The sp0987 gene in the S. pneumoniae TIGR4 strain encodes a putative single-domain protein belonging to the GH25 family. As mutational analysis indicated that this novel protein might be involved in host-cell invasion, we named this protein Glycosyl Hydrolase 25 relating to Invasion Protein (GHIP). GHIP is a novel type of GH25 protein containing a single-domain catalytic module, which differs from other known GH25 that contain at least two distinct domains, including a catalytic module and a choline-binding module. Functionally, GHIP can hydrolyze peptidoglycan using the active site located at the mouth of its barrel structure; in addition, deleting the GHIP gene has a strongly inhibits S. pneumoniae virulence.

Therefore, in order to better understand the function of this novel virulence factor, we elucidated and now report the X-ray structure of GHIP at 1.86 Å resolution. The GHIP crystal structure was phased by single-wavelength anomalous dispersion at 3.0 Å resolution and refined against the diffraction data acquired from the native GHIP crystal at 1.86 Å with a 24.5% free R-factor and an 18.0% crystallographic R-factor. The final model consisted of 227 amino acids (residues 15–243) and 200 water molecules. Due to conformational disorder, the N-terminal residues (1–14) were not represented in the electron density and therefore not included in the final model. Only one GHIP molecule was present in the asymmetric unit. The overall structure of GHIP consists of one domain shaped into a flattened ellipsoid with dimensions of 30 Å × 38 Å × 40 Å. GHIP contains an inner ring of seven parallel β-sheets (β1–7) with a protruding β-strand (β8) at the C-terminal region, and an outer wheel composed of eight α-helices surrounds this inner ring. 14 amino acids, including Asp56, Ser58, Ser84, Tyr121, Tyr123, Glu154, Glu156, Asp157, Tyr185, Tyr209, Asp212, Ser233, Asp243, and Asp245, form a negatively charged groove at the mouth of the GHIP barrel. Analogously, the four corresponding residues in GHIP homologs, including Asp56, Asp154, Glu156, and Asp245, are also strictly conserved. All mutants showed lower hydrolytic activity compared to wild-type GHIP, suggesting that these four residues are located at the active site of this novel peptidoglycan hydrolase enzyme.

> MRKQIHPLILFSFFGIMMFILIINRPLNDSQSFKTKSNIAQIEAQALKHLDKPIIDLSGWQRPEEINYDALSQNISGAIVRVHSGAQTTKENDASFINGIDKAYKSHITELQKRNVPVAVYAYVAGKSVQEMEKAAEVFYNAASPYSPSYYWLDVEDKTMSNMNEGVENFRAKLASLGAKNIGIYVGVYFMEEHSIDTGKFTSVWIPSYGSDSGFLESSPKTDLDYDIHQYTSKGKIAGFDHDLDINVISPLKNKEETFRKLFLKP[(1R,3R,4R,7S)-7-HYDROXY-3-(5-METHYLCYTOSIN-1-YL)-2,5-DIOXABICYCLO[2.2.1]HEPT-1-YL]METHYL DIHYDROGEN PHOSPHATE 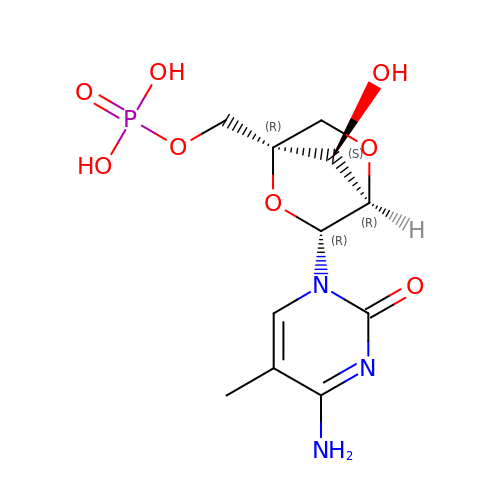| C11 H16 N3 O8 P | RSSHBVFUGGVGMZ-YRCORFKGSA-N> MGIPAAFRWLSNKYPKIISPVVEERPIVMPDGTEIPVDATRPNPNGEEFDNLYLDMNGIVHPCSHPEDKPAPKDEEEMMIEIFKYTDRIVKMVRPRKILMIAVDGVAPRAKMNQQRSRRFRAAQEAKEKEEEKKQLLKMLRKEKGSNMQEEPLETVVKKAFDSNSITPGTPFMDILAASLRYWCAYKLNTDPAWAKLKVIISDATVPGEGEHKIMEFIRSQRSSPEHNPNTRHVIYGLDADLIMLGLATHEPHFRVLREDVFFQEAKARLCKLCGQKGHDERSCKGEAKQKQGEFDEKDHAQPLKPFIWLHVSILREYLAAELEVPNLPFRWDLERAIDDWVFLCFFVGNDFLPHLPALEIRENGIDTLTAIWKDNLPIMGGYLTKDGHVDLERAQYILNGLAKQEDAIFRRRREVEERREANAKRRKLNQQGAHAKGAADSHAGKSGRKHVPEAAGPLPGMALFPITNPPPPAITHDMVMKGRSVDQANLANKSAASVLKSQIQSMMAQKAATNANGAEKDVSADGTTTAPASALGKRKAELIEEDAATNTDTDSVTDGTGSDNEGPVDTVRLWEEGYADRYYEQKFKVDPKDIEFRHKVGRAYAEGLAWVLQYYYQGCPSWEWFYPYHYAPFAADFVDLAKMEIKFEKGRISRPFEQLMSVLPAASRHAIPEVYHDLMTDPNSPIIDFYPEEFEIDLNGKKMAWQGVALLPFIEMPRLLAAMKEREHLLSEEDRARNEPGFDVLLISDAHPGLYEDITSHFYSKKQGAPKFKLNPRRSDGLAGKVEKIEGYVPHGSLVYPLARNSMPDVDYDRSITVRYIMPSSAHQHKSMLLRGVKLPPPALSRSDIEIIRSKAKNAGRSYGGAPLRNNYNSLEHHHHHH

In this work, we studied the structure and dynamics of the essential 100-kDa eukaryotic 5′→3′ exoribonuclease Xrn2. The molecular basis of RNA degradation by Xrn2 and its cytoplasmic paralogue Xrn1 has been established by several studies. Both enzymes are highly selective for substrates with exposed 5′-monophosphorylated ends and require divalent cations to catalyze the hydrolysis of phosphodiester bonds. On a structural level, Xrn1 and Xrn2 share two conserved regions (CR1 and CR2) and a less conserved C-terminal segment (CTS), which together form the Xrn core domain. This Xrn core harbors the catalytic site, which has three crucial features.

Here, we found that the Xrn2 core from the thermophilic yeast Chaetomium thermophilum (CtXrn2, residues 1–875, molecular weight 100 kDa) fulfills those conditions. To lay the structural foundation for our NMR experiments, we first determined the crystal structure of CtXrn2. The active site of the enzyme is positioned in a pocket in front of the ‘tower’ domain helix (helix α4). Seven acidic residues provide a coordination platform for the two catalytically important Mg2+ ions. In our structure of the Xrn2 enzyme, electron density is lacking for three regions: (1) the top of the tower domain (residues 135–158) that is also less well defined in other Xrn2 structures; (2) the linker region between CR1 and CR2 (residues 423–568) that is highly flexible in solution; and (3) a short loop between residues 266 and 304 that harbors a putative CCHC zinc finger (ZnF) motif. However, in our crystal structure of apo CtXrn2, this XTBD segment is already fully folded, and the chemical shifts of Ile687 and Ile688 δ1-methyl groups clearly deviate from the shift of Ileδ1-methyl groups in unstructured regions. The precision of the extracted population is limited, as can be judged from the shallow minimum in the reduced χ2 surface. Taken together, our data establish that the α1-‘ratchet’-helix of Xrn2 samples multiple states in solution in the absence of a substrate, whereas other parts of the enzyme are largely devoid of motions on the millisecond time scale Fig. 2 Methyl-TROSY NMR reveals conformational dynamics located around the N-terminal α1-helix. In summary, our data reveal that the apo Xrn2 enzyme is in a dynamic equilibrium between the pre-translocation and post-translocation states.>[2x]MIERLNSPFLRAAALFTIVAFSSLISTAALAENNPSDTAKKFKVVTTFTIIQDIAQNIAGDVAVVESITKPGAEIHDYQPTPRDIVKAQSADLILWNGMNLERWFEKFFESIKDVPSAVVTAGITPLPIREGPYSGIANPHAWMSPSNALIYIENIRKALVEHDPAHAETYNRNAQAYAEKIKALDAPLRERLSRIPAEQRWLVTSEGAFSYLAKDYGFKEVYLWPINAEQQGI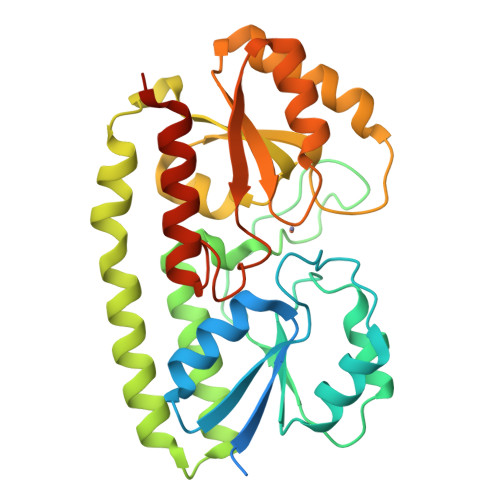PQQVRHVIDIIRENKIPVVFSESTISDKPAKQVSKETGAQYGGVLYVDSLSGEKGPVPTYISLINMTVDTIAKGFGQLEHHHHHHHHHH>[2x]MSKTQEFRPLTLPPKLSLSDFNEFIQDIIRIVGSENVEVISSKDQIVDGSYMKPTHTHDPHHVMDQDYFLASAIVAPRNVADVQSIVGLANKFSFPLWPISIGRNSGYGGAAPRVSGSVVLDMGKNMNRVLEVNVEGAYCVVEPGVTYHDLHNYLEANNLRDKLWLDVPDLGGGSVLGNAVERGVGYTPYGDHWMMHSGMEVVLANGELLRTGMGALPDPKRPETMGLKPEDQPWSKIAHLFPYGFGPYIDGLFSQSNMGIVTKIGIWLMPNPRGYQSYLITLPKDGDLKQAVDIIRPLRLGMALQNVPTIRHILLDAAVLGDKRSYSSRTEPLSDEELDKIAKQLNLGRWNFYGALYGPEPIRRVLWETIKDAFSAIPGVKFYFPEDTPENSVLRVRDKTMQGIPTYDELKWIDWLPNGAHLFFSPIAKVSGEDAMMQYAVTKKRCQEAGLDFIGTFTVGMREMHHIVCIVFNKKDLIQKRKVQWLMRTLIDDC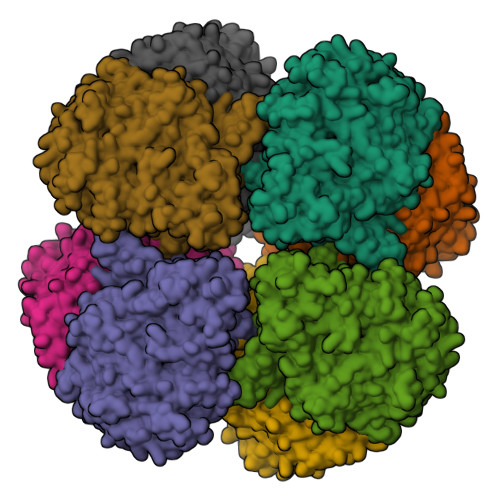AANGWGEFRTHLAFMDQIMETYNWNNSSFLRFNEVLKNAVDPNGIIAPGKSGVWPSQYSHVTWKL>MTRRVAIGTDHPAFAIHENLILYVKEAGDEFVPVYCGPKTAESVDYPDFASRVAEMVARKEVEFGVLAAGSGIGMSIAANKVPGVRAALCHDHYTAAMSRI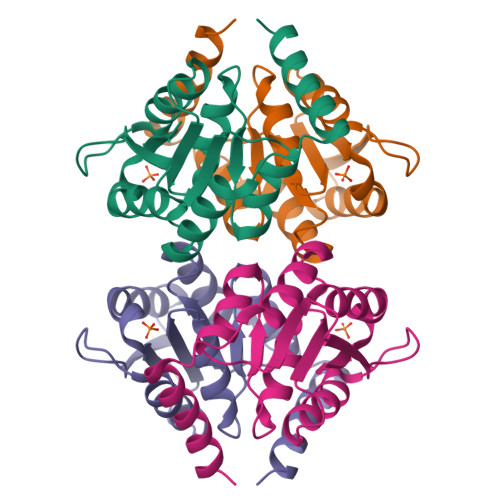HNDANIVCVGERTTGVEVIREIIITFLQTPFSGEERHVRRIEKIRAIEASHA[2x]> MRGSHHHHHHGSMPETNPNAPPRPDSLLNPSDALKHLEEYPRGDGLSLQE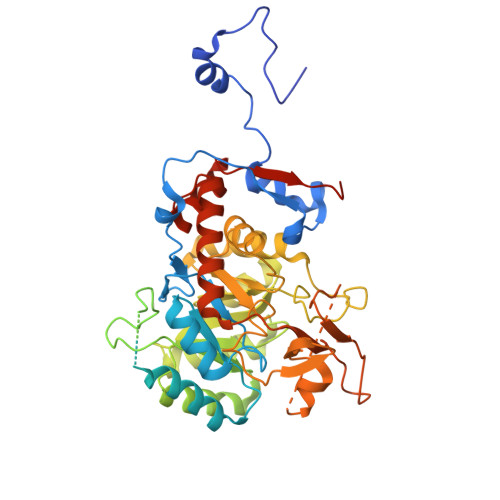LMDSRKNGGLTYNDFLVLPGHINFPASDVSLQSKATKNIVLNTPFLSSPMDTVTEDRMAIALALHGGLGIIHHNCSAEEQAAMVRRVKKYENGFITDPLCLGPDATVGDVLEIKAKFGFCGVPITETGEPDSKLLGIVTGRDVQFQDAETPIKSVMTTEVVTGSSPITLEKANSLLRETKKGKLPIVDSNGHLVSLVARSDLLKNQNYPYASKVPESKQLYCGAAIGTRPGDKDRLKLLAEAGLDVVVLDSSQGNSVYQIEFIKWIKQTYPKIDVIAGNVVTREQAAQLIAAGADGLRIGMGSGSICITQEVMAVGRPQGTAVYAVAEFASRFGIPCIADGGIGNIGHIAKALALGASAVMMGGLLAGTTESPGEYFYHEGKRVKVYRGMGSIEAMEHTQRGSASGKRSILGLDNAATARYFSEADAVKVAQGVSGDVADKGSINKFVPYLFTGLQHSLQDAGIKSVSELHSCARSGSLRFELRTASAQLEGGVHGLNSYTKRLFA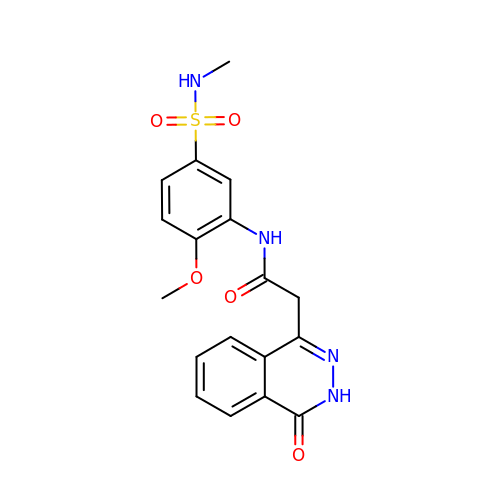~{N}-[2-methoxy-5-(methylsulfamoyl)phenyl]-2-(4-oxidanylidene-3~{H}-phthalazin-1-yl)ethanamide | C18 H18 N4 O5 S | GSAOPHWPZFNUCK-UHFFFAOYSA-N>SGTTEKTVAKEEKVKLTDQ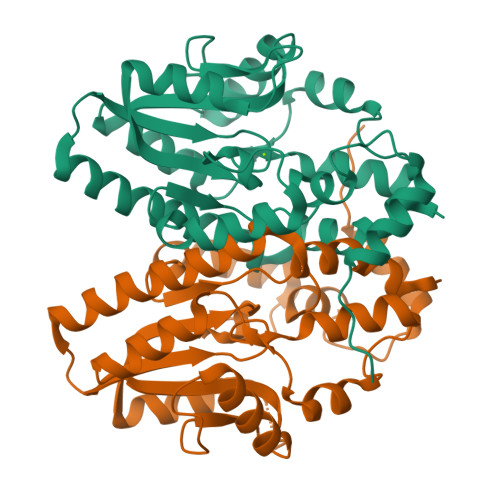QLMADLWYQTAGEMKALYYQGYNTGQLKLDAALAKGTEKKPAIVLDLDETVLDNSPHQAMSVKTGKGYPYKWDDWINKAEAEALPGSIDFLKYTESKGVDIYYISNRKTNQLDATIKNLERVGAPQATKEHILLQDPKEKGKEKRRELVSQTHDIVLFFGDNLSDFTGFDGKSVKDRNQAVTDSKAQFGEKFIIFPNPMYGDWEGALYDYNFKKSDAEKDKIRHDNLKSFDAKHHHHHH[2x]> ML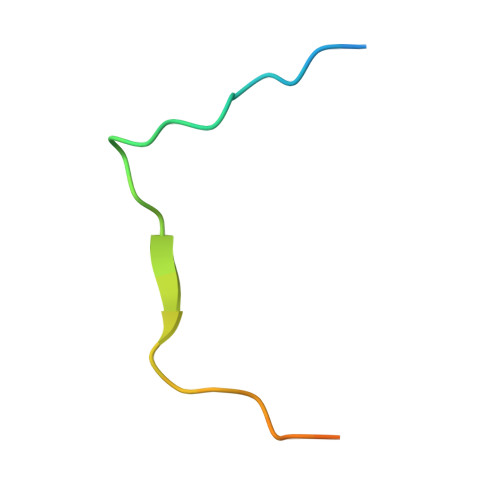SRFIPWFPYDGSKLPLRPKRSPPASREEIMATL>GGAPWQAEEWYFGKITRRESERLLLNAENPRGTFLVREGQS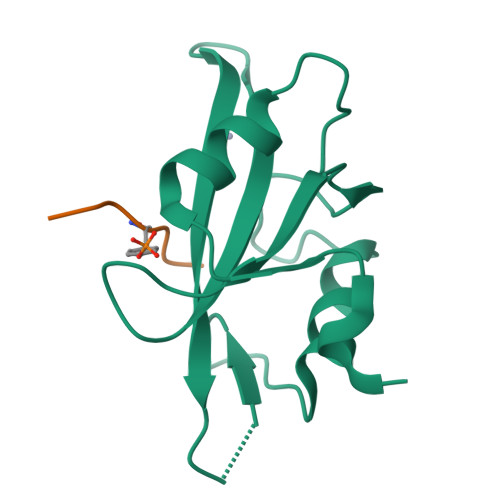QPDYVLSVSDFDNAKGLNVKHYIIRKLDSGGFYITSRTQFNSLQQLVAYYSKHADGLCHRLTTVCPTSRA[2x];>EPQYEEI[2x]> SMAAAGPGKTSW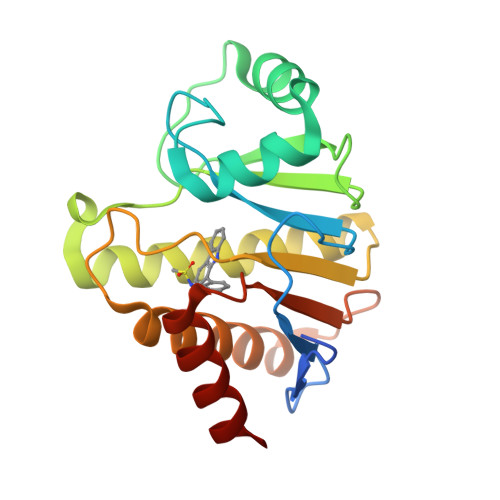EKGSLVSPGGLQMLLVKEGVQNAKTDVVVNSVPLDLVLSRGPLSSSLLEKAGPELQEELDTVGQGVAVSMGTVLKTSSWNLDCRYVLHVVAPEWRNGSTSSLKIMEDIIRECMEITESLSLKSIAFPAIGTGNLGFPKNIFAELIISEVFSFSSSNQLSTLQEVHFLLHPSDHENIQAFSDEFARRAN> GSIGAPNTTFGTNNHHLYPDELNVSNNPHYRPKPVSYDSTLPPDHIKVYSRTLFIGGVPLNMKEWDLANVLKPFAEVQSVILNNSRKHAFVKVYSRHEAENVLQNFNKDGALPLRTRWGVGFGPRDCCDYQHGYSIIPMHRLTDADKKWSVSAQWGGTSGQPLVTGIVFEEP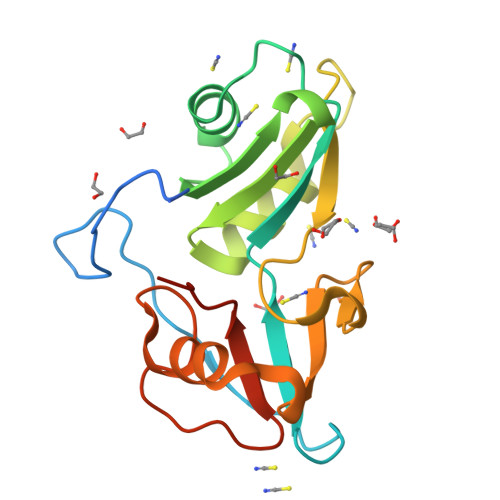DIIVGEGV>MYHCHSGSKPTEKGANEYAYAKWKLCSASAIC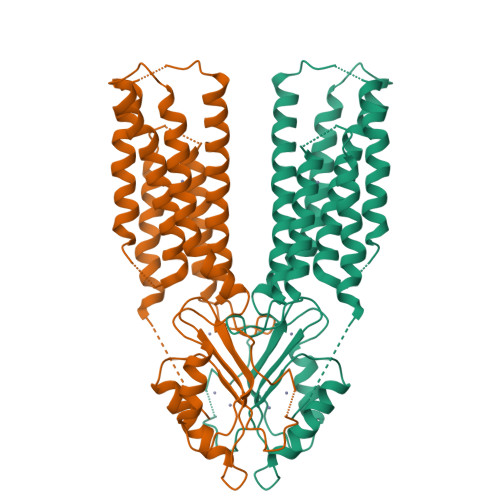FIFMIAEVVGGHIAGSLAVVTDAAHLLIDLTSFLLSLFSLWLSSKPPSKRLTFGWHRAEILGALLSILCIWVVTGVLVYLACERLLYPDYQIQATVMIIVSSCAVAANIVLTVVLHQRCLGHNHKEVQANASVRAAFVHALGDLFQSISVLISALIIYFKPEYKIADPICTFIFSILVLASTITILKDFSILLMEGVPKSLNYSGVKELILAVDGVLSVHSLHIWSLTMNQVILSAHVATAASRDSQVVRREIAKALSKSFTMHSLTIQMESPVDQDPDCLFCEDPCD[2x]RNA polymerase III (Pol III) transcribes a number of abundant, short, folded RNAs in the eukaryotic cell, including tRNAs, 5 S rRNA, spliceosomal U6 RNA, and the signal recognition particle 7SL RNA. In yeast, transcription of all Pol III genes minimally requires two conserved transcription factors (TFs) to initiate transcription in vivo, namely TFIIIC and TFIIIB. cerevisiae TFIIIC consists of six subunits with a combined molecular weight of 520 kDa, and binds to promoter elements termed A-box and B-box that are downstream of the transcription start site (TSS). The six subunits of TFIIIC are organized in two subcomplexes: τA comprises subunit τ131, τ95, and τ55, and τB comprises subunits τ138, τ91, and τ60. τA binds the A-box with low affinity and is responsible for TFIIIB recruitment. τB binds the B-box with high affinity, and the quality of the B-box determines promoter strength.

We report a 3.1 Å cryo-electron microscopy (cryo-EM) structure of τA, which constitutes the most conserved part of TFIIIC. We collected cryo-EM data of a sample containing τA, TFIIIB, and a DNA fragment comprising the A-box and the TFIIIB-binding promoter elements of the His_tH(GUG)E2 gene. However, TFIIIB and DNA had dissociated from τA during sample preparation and are not visible in the EM density. The cryo-EM map allowed us to build an atomic model of τA with excellent refinement statistics, but also revealed density for two molecules of the detergent CHAPSO, which was added before plunge-freezing to prevent adsorption to the air–water interface, bound to τA. Interestingly, our cryo-EM map reveals a molecule of the detergent CHAPSO bound to the right arm of τ131, which is also predicted to bind TFIIIB, and it is therefore possible that addition of CHAPSO competed with TFIIIB for binding to τ131 and thereby contributed to dissociation of TFIIIB from τA. The convex surface of the N-terminal τ131 TPR array binds the τ55 HPD and the triple β-barrel formed by the τ55–τ95 dimerization domains. Despite only being present in hemiascomycetes and being absent in other eukaryotes, the τ55 HPD is well-ordered and an integral part of the τA structure, rather than being flexibly attached to the τA core. Our structure shows that the τ55 active site is accessible in τA, arguing that TFIIIC can directly modify substrates and the activity might be coupled to its function as a TF. The acidic plug contains a helix that is rich in negatively charged residues and is embedded in the positively charged DBD.

> MAAGKLKKEQQNQSAERESADTGKVNDEDEEHLYGNIDDYKHLIQDEEYDDEDVPHDLQLSEDEYNSERDSSLLAEFSDYGEISEDDEEDFMNAIREASNFKVKKKKKNDKGKSYGRQRKERVLDPEVAQLLSQANEAFVRNDLQVAERLFNEVIKKDARNFAAYETLGDIYQLQGRLNDCCNSWFLAAHLNASDWEFWKIVAILSADLDHVRQAIYCFSRVISLNPMEWESIYRRSMLYKKTGQLARALDGFQRLYMYNPYDANILRELAILYVDYDRIEDSIELYMKVFNANVERREAILAALENALDSSDEESAAEGEDADEKEPLEQDEDRQMFPDINWKKIDAKYKCIPFDWSSLNILAELFLKLAVSEVDGIKTIKKCARWIQRRESQTFWDHVPDDSEFDNRRFKNSTFDSLLAAEKEKSYNIPIDIRVRLGLLRLNTDNLVEALNHFQCLYDETFSDVADLYFEAATALTRAEKYKEAIDFFTPLLSLEEWRTTDVFKPLARCYKEIESYETAKEFYELAIKSEPDDLDIRVSLAEVYYRLNDPETFKHMLVDVVEMRKHQVDETLHRISNEKSSNDTSDISSKPLLEDSKFRTFRKKKRTPYDAERERIERERRITAKVVDKYEKMKKFELNSGLNEAKQASIWINTVSELVDIFSSVKNFFMKSRSRKFVGILRRTKKFNTELDFQIERLSKLAEGDSVFEGPLMEERVTLTSATELRGLSYEQWFELFMELSLVIAKYQSVEDGLSVVETAQEVNVFFQDPERVKMMKFVKLAIVLQMDDEEELAENLRGLLNQFQFNRKVLQVFMYSLCRGPSSLNILSSTIQQKFFLRQLKAFDSCRYNTEVNGQASITNKEVYNPNKKSSPYLYYIYAVLLYSSRGFLSALQYLTRLEEDIPDDPMVNLLMGLSHIHRAMQRLTAQRHFQIFHGLRYLYRYHKIRKSLYTDLEKQEADYNLGRAFHLIGLVSIAIEYYNRVLENYDDGKLKKHAAYNSIIIYQQSGNVELADHLMEKYLSIRSGG;> MHHHHHHENLYFQSMPVEEPLATLSSIPDSSADQAPPLIADEFTLDLPRIPSLELPLNVSTKHSSIQKAIKMCGGIEKVKEAFKEHGPIESQHGLQLYLNDDTDSDGSKSYFNEHPVIGKRVPFRDESVILKVTMPKGTLSKNNNSVKDSIKSLKDSNKLRVTPVSIVDNTIKFREMSDFQIKLDNVPSAREFKSSFGSLEWNNFKSFVNSVPDNDSQPQENIGNLILDRSVKIPSTDFQLPPPPKLSMVGFPLLYKYKANPFAKKKKNGVTEVKGTYIKNYQLFVHDLSDKTVIPSQAHEQVLYDFEVAKKTKVYPGTKSDSKFYESLEECLKILRELFARRPIWVKRHLDGIVPKKIHHTMKIALALISYRFTMGPWRNTYIKFGIDPRSSVEYAQYQTEYFKIERKLLSSPIVKKNVPKPPPLVFESDTPGGIDSRFKFDGKRIPWYLMLQIDLLIGEPNIAEVFHNVEYLDKANELTGWFKELDLVKIRRIVKYELGCMVQGNYEYNKYKLKYFKTMLFVKESMVPENKNSEEGMGVNTNKDADGDINMDAGSQMSSNAIEEDKGIAAGDDFDDNGAITEEPDDAALENEEMDTDQNLKVPASIDDDVDDVDADEEEQESFDVKTASFQDIINKIAKLDPKTAETMKSELKGFVDEVDLXXXXXXXXXXXXXXXXXXXXXX;> MVVNTIYIARHGYRSNWLPEGPYPDPLTGIDSDVPLAEHGVQQAKELAHYLLSLDNQPEAAFASPFYRCLETVQPIAKLLEIPVYLERGIGEWYRPDRKPVIPVPAGYEILSKFFPGVISQEWDSTLTPNEKGETEQEMYMRFKKFWPLFIERVEKEYPNVECILLVTHAASKIALGMSLLGYDNPRMSLNENGDKIRSGSCSLDKYEILKKSYDTIDETDDQTSFTYIPFSDRKWVLTMNGNTEFLSSGEEMNWNFDCVAEAGSDADIKKRQMTKKTSSPIPEADDQTEVETVYISVDIPSGNYKERTEIAKSAILQYSGLETDAPLFRIGNRLYEGSWERLVGTELAFPNAAHVHKKTAGLLSPTEENETTNAGQSKGSSTANDPNIQIQEEDVGLPDSTNTSRDHTGDKEEVQSEKIYRIKERIVLSNVRPM> MHHHHHHMTMDEQQSQAVAPVYVGGFLARYDQSPDEAELLLPRDVVEHWLHAQGQGQPSLSVALPLNINHDDTAVVGHVA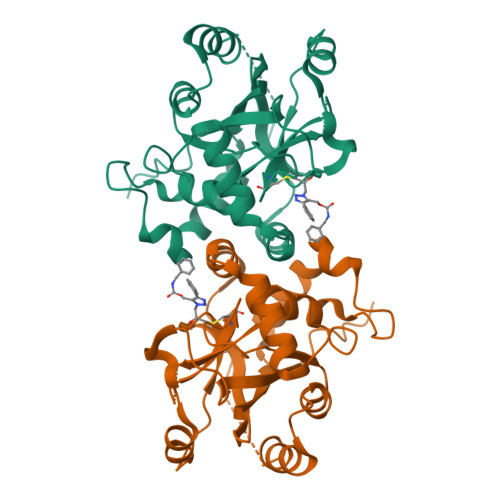AMQSVRDGLFALGAVTSPRFLEIVRRASEKSELVSRGPVSPLQPDKVVEFLSGSYAGLSLSSRRADDVEVATSLSGSETTPFKHVALCSVGRRRGTLAVYGRDPEWVTQRFPDLTAADRDGLRAQWQRAGSTAVDVSGDPFRSDSYGLLGNSVDALYIRERLPKLRYDKQLVGVTERESYVKA>MAAKLWTFLLGFGLSWVWPASAHRKLLVLLLDGFRSDYISEDALASLPGFREIVNRGVKVDYLTPDFPSLSYPNYYTLMTGRHCEVHQMIGNYMWDPRTNKSFDIGVNRDSLMPLWWNGSEPLWITLMKARRKVYMYYWPGCEVEILGVRPTYCLEYKTVPTDINFANAVSDALDSLKSGRADLAAIYHERIDVEGHHYGPSSPQRKDALRAVDTVLKYMIQWIQDRGLQQDLNVILFSDHGMTDIFWMDKVIELSNYISLDDLQQVKDRGPVVSLWPVPGKHSEIYHKLRTVEHMTVYEKESIPNRFYYKKGKF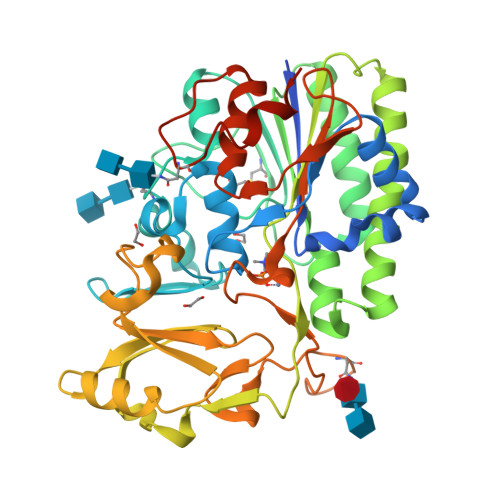VSPLTLVADEGWFIAESREMLPFWMNSTGKREGWQRGWHGYDNELMDMRGIFLAIGPDFKSNFRAAPIRSVDVYNIMAHVAGITPLPNNGSWSRVVSMLKGQTSSASRENLYFQ[2x]> MAPLIVVTGLPSSGKTTRARQLYAYLEERIASQPKSQMPSQPQPQHPPQSQPPSQSQTSPIPPPLSSTPQYRLHYISDATLSISRSVYDLSPEKLPAHVRSANASEKDARAALYAAVKRVLGPKDIVILDSLNYIKGWRYQLYCEAKNARTPSCVLQVGGGVEKAREVNERRLERRERKLKEQGEKKEGEEKKEAAESDEEPYERSNWENLVFRYEEPNPMTRWDSPLFLLAWDDDEAQTRQ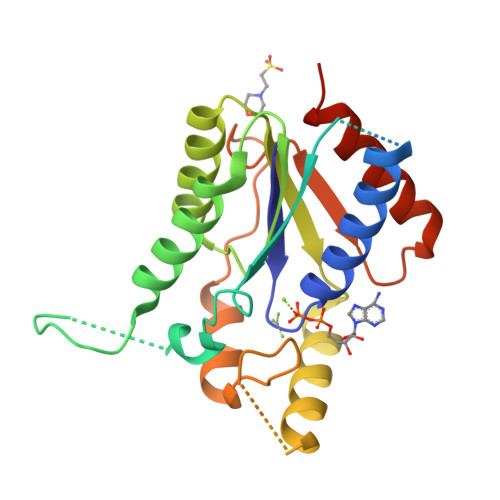VFDKIWDAIAGEGLEHHHHHH>GPGSMTIIEVKIKKLENFLGNLPEYATEHSAGMDLVAANEQSITIKVGSIQLIPTGIAIALPESFEAQIRPRSGLAVKHGITVANSPGTIDADYRGEIKVLLINLGNKDFIIEKGMRIAQMIIAKYERV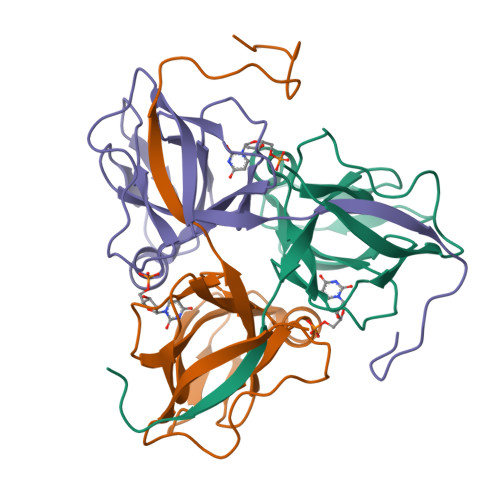LWAETSILTETMRGRGGFGSTGL[6x]> MRGSHHHHHHGIRMTRISREMMKELLSVYFIMGSNNTKADPVTVVQKALKGGATLYQFREKGGDALTGEARIKFAEKAQAACREAGVPFIVNDDVELALNLKADGIHIGQEDANAKEVRAAIGDMILGVSAHTMSEVKQAEEDGADYVGLGPIYPTETKKDTRAVQGVSLIEAVRRQG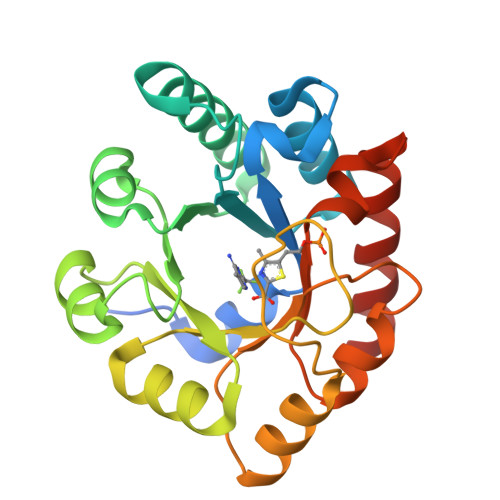ISIPIVGIGGITIDNAAPVIQAGADGVSMISAISQAEDPESAARKFREEIQTYKTGR> 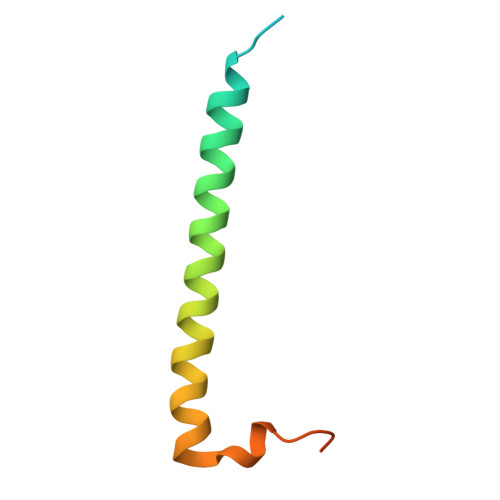MSDPAFAYAQLTHDELIQLVLKQKETISKKEFQVRELEDYIDNLLVRVMEETPNILRIPTQVGKKAGKM>GTGAMIVKPMVRNNICLNAHPQGCKKGVEDQIEYTKKRITAEVKAGAKAPKNVLVLGCSNGYGLASRITAAFGYGAATIGVSFEKAGSETKYGTPGWYNNLAFDEAAKREGLYSVTIDGDAFSDEIKAQVIEEAKKKGIKFDLIVYSLASPVRTDPDTGIMHKSVLKPFGKTFTGKTVDPFTGELKEISAEPANDEEAAATVKVMGGEDWERWIKQLSKEGLLEEGCITLAYSYIGPEATQALYRKGTIGKAKEHLEATAHRLNKENPSIRAFVS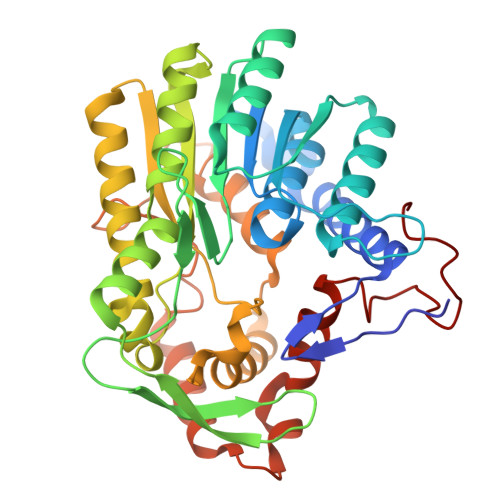VNKGLVTRASAVIPVIPLYLASLFKVMKEKGNHEGCIEQITRLYAERLYRKDGTIPVDEENRIRIDDWELEEDVQKAVSALMEKVTGENAESLTDLAGYRHDFLASNGFDVEGINYEAEVERFDRI[4x]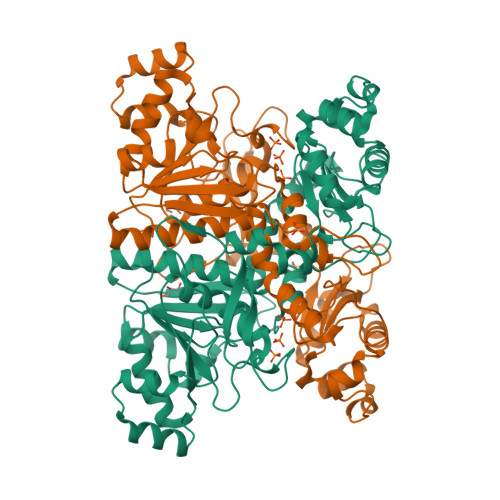>[2x]SYYHHHHHHLESTSLYKKAGLMSTPLQGIKVLDFTGVQSGPSCTQMLAWFGADVIKIERPGVGDVTRHQLRDIPDIDALYFTMLNSNKRSIELNTKTAEGKEVMEKLIREADILVENFHPGAIDHMGFTWEHIQEINPRLIFGSIKGFDECSPYVNVKAYENVAQAAGGAASTTGFWDGPPLVSAAALGDSNTGMHLLIGLLAALLHREKTGRGQRVTMSMQDAVLNLCRVKLRDQQRLDKLGYLEEYPQYPNGTFGDAVPRGGNAGGGGQPGWILKCKGWETDPNAYIYFTIQEQNWENTCKAIGKPEWITDPAYSTAHARQPHIFDIFAEIEKYTVTIDKHEAVAYLTQFDIPCAPVLSMKEISLDPSLRQSGSVVEVEQPLRGKYLTVGCPMKFSAFTPDIKAAPLLGEHTAAVLQELGYSDDEIAAMKQNHAI> MDPEEILERAKESLERAREASERGDEEEFRKAAEKALELAKRLVEQAKKEGDPELVLEAAKVALRVAELAAKNGDKEVFKKAAESALEVAKRLVEVASKEGDPELVLEAAKVALRVAELAAKNGDKEVFKKAAESA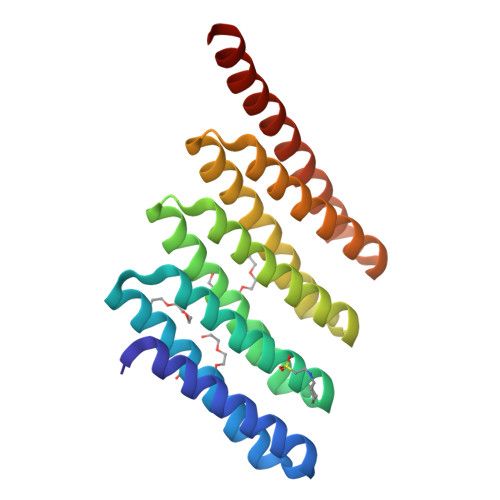LEVAKRLVEVASKEGDPELVEEAAKVAEEVRKLAKKQGDEEVYEKARETAREVKEELKRVREEKGGWLEHHHHHH>[2x]MTLYSCCLILLLFTWNTAAYGPNQRAQKKGDIILGGLFPIHFGVAAKDQDLKSRPESVECIRYNFRGFRWLQAMIFAIEEINNSPNLLPNMTLGYRIFDTCNTVSKALEATLSFVAQNKIDSLNLDEFCNCSEHIPSTIAVVGATGSGVSTAVANLLGLFYIPQVSYASSSRLLSNKNQFKSFLRTIPNDEHQATAMADIIEYFRWNWVGTIAADDDYGRPGIEKFREEAEERDICIDFSELISQYSDEEEIQQVVEVIQNSTARVIVVFSSGPDLEPLIKEIVRRNITGKIWLASEAWASSSLIAMPEFFRVIGSTIGFALKAGQIPGFREFLQKVHPKKSANNGFAKEFWEETFNCYLPSESKNSPASASFHKAHEEGLGAGNGTAAFRPPCTGDENITSVETPYMDFTHLRISYNVYLAVYSIAHALQDIYTCTPGKGLFTNGSCADIKKVEAWQVLKHLRHLNFT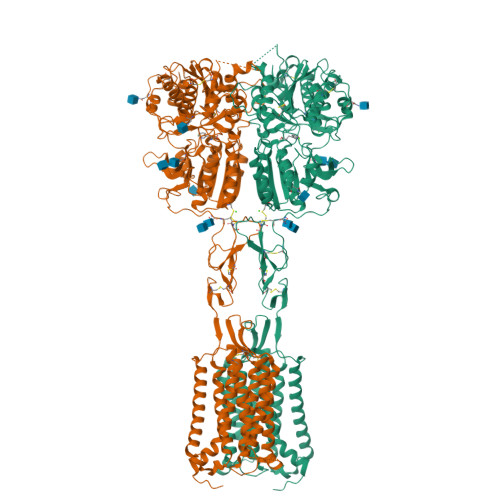SNMGEQVDFDEFGDLVGNYSIINWHLSPEDGSVVFEEVGHYNVYAKKGERLFINENKILWSGFSKEVPFSNCSRDCLPGTRKGIIEGEPTCCFECVDCPDGEYSDETDASACDKCPEDYWSNENHTSCIPKQIEFLSWTEPFGIALTLFAVLGIFLTSFVLGVFTKFRNTPIVKATNRELSYLLLFSLLCCFSSSLFFIGEPQNWTCRLRQPAFGISFVLCISCILVKTNRVLLVFEAKIPTSLHRKWWGLNLQFLLVFLCTFVQIVICVIWLYTAPPSSYRNHELEDEIIFITCHEGSLMALGFLIGYTCLLAAICFFFAFKSRKLPENFNEAKFITFSMLIFFIVWISFIPAYASTYGKFVSAVEVIAILAASFGLLACIFFNKVYIILFKPSRNTIEEVRCSTAAHAFKVAARATLRRSNVSRKRSNSLGGSTGSTPSSSISSKSNHEDPFPLPASAERQRQQQRGCKQKVSFGSGTVTLSLSFEEPQKNAMANRNAKRRNSLEAQNSDDSLMRHRALLALQNSESLSAEPGFQTASSPETSSQESVVGDNKEEVPNPEAEPSLPSANSRNFIGTGGSSVTENTVHSLESALEVLFQ(3R,4S,5S)-3-[(3-tert-butylbenzyl)amino]-5-{[3-(2,2-difluoroethyl)-1H-indol-5-yl]methyl}tetrahydro-2H-thiopyran-4-ol 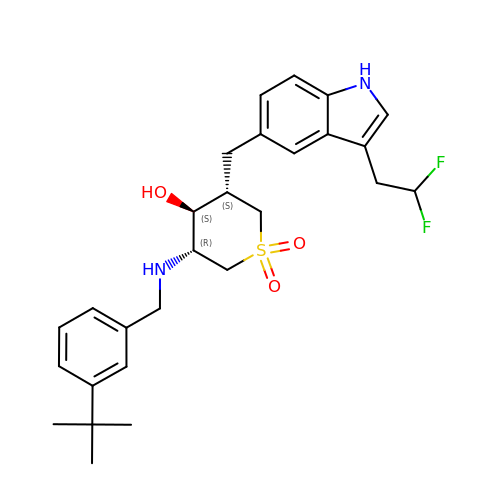1,1-dioxide | C27 H34 F2 N2 O3 S | OOZZVYSXZBAROL-PSUQPPDWSA-N> MVKLMIIEGEVVSGLGEGRYFLSLPPY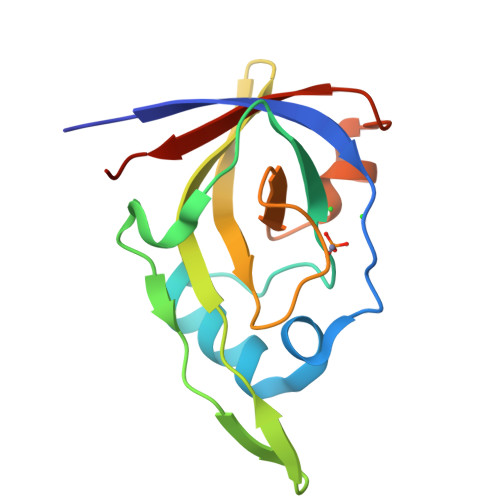KEIFKKILGFEPYEGTLNLKLDREFDINKFKYIETEDFEFNGKRFFGVKVLPIKILIGNKKIDGAIVVPKKTYHSSEIIEIIAPMKLREQFNLKDGDVIKILIKGDKDE>[2x]SELIVNVINGPNLGRLGRREPAVYGGTTHDELVALIEREAAELGLKAVVRQSDS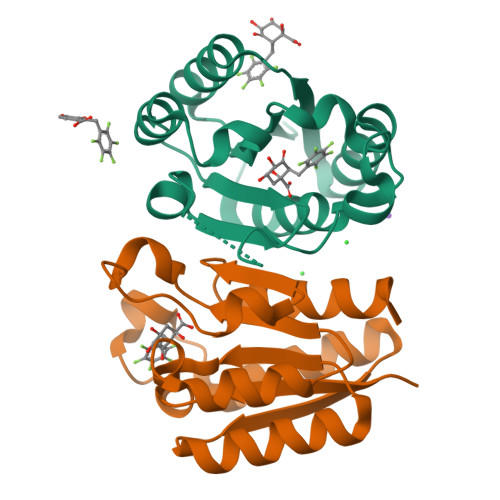EAQLLDWIHQAADAAEPVILNAGGLTHTSVALRNACAELSAPLIEVHISNVHAREEFRRHSYLSPIATGVIVGLGIQGYLLALRYLAEHVGT>[2x]MAAEDFLTIFLDDDESWNETLNMSGYDYSGNFSLEVSVCEMTTVVPYTWNVGILSLIFLINVLGNGLVTYIFCKHRSRAGAIDILLLGICLNSLCLSISLLAEVLMF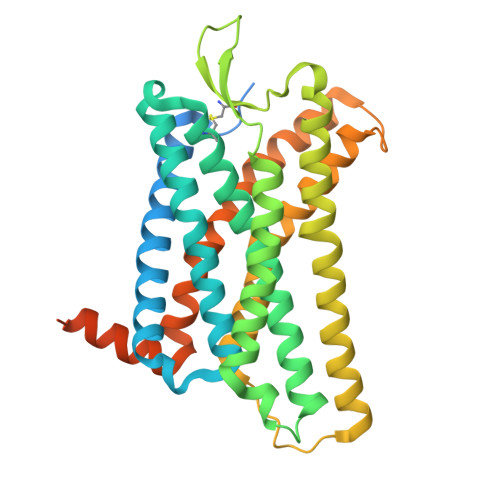LFPNIISTGLCRLEIFFYYLYVYLDIFSVVCVSLVRYLLVAYSTRSWPKKQSLGWVLTSAAWLIALVLSGDACRHRSRVVDPVSKQAMCYENAGNMTADWRLHVRTVSVTAGFLLPLALLILFYALTWCVVRRTKLQARRKVRGVIVAVVVLFFVFCFPYHVLNLLDTLLRRRWIRDSCYTRGLINVGLAVTSLLQALYSAVVPLIYSCLGSLFRQRMYGLFQSLRQSFMSGADYKDDDDKGRPLEVLFQGPHHHHHHHHHH>SHM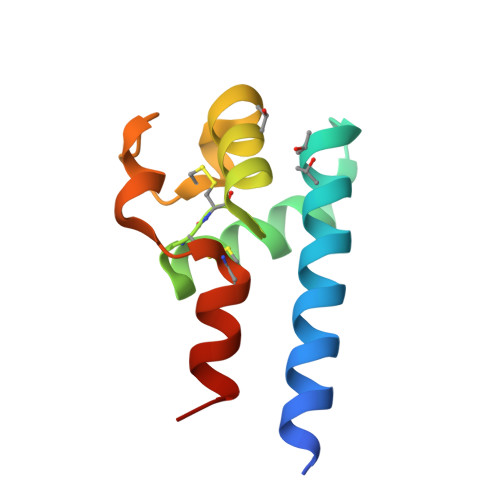FVNKDQIAKDVKQFYDQALQQAVMDDDANNAKAVVKTFHETLNCCGSNALTTLTTTILRNSLCPSGGNILTPLLQQDCHQKIDELFSGKL[2x]3-cyclopropyl-4-(furan-2-yl)-1H-pyrazolo[3,4-b]pyridine 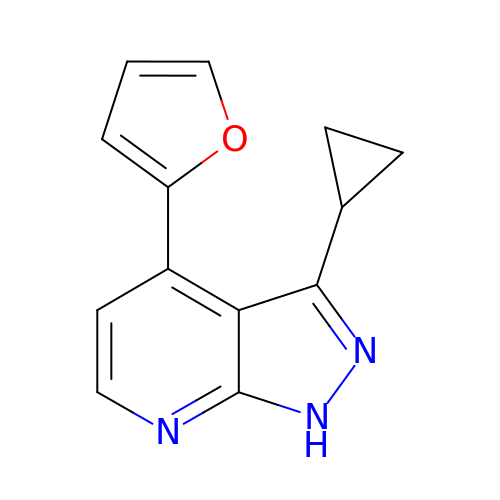| C13 H11 N3 O | CVODVHVJEVVKKB-UHFFFAOYSA-N>[2x]TKDKYRVVYTDHQRLELEKEFHYSRYITIRRKAELAATLGLSERQVKIWF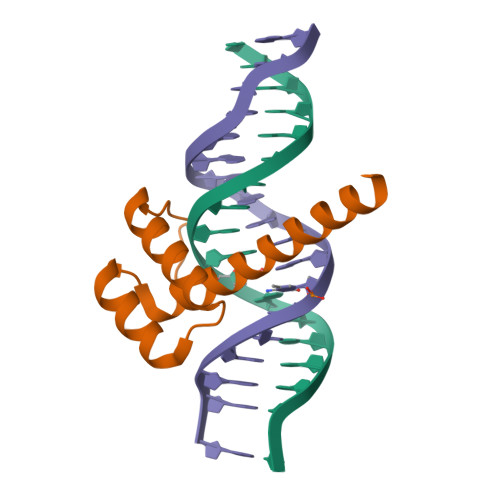QNRRAKERKINKKKLQQQQQQ> MAAQGFLLIATFLLVLMVLARPLGSGLARLINDIPLPGTTGVERVLFRALGVSDREMNWKQYLCAILGLNMLGLAVLFFMLLG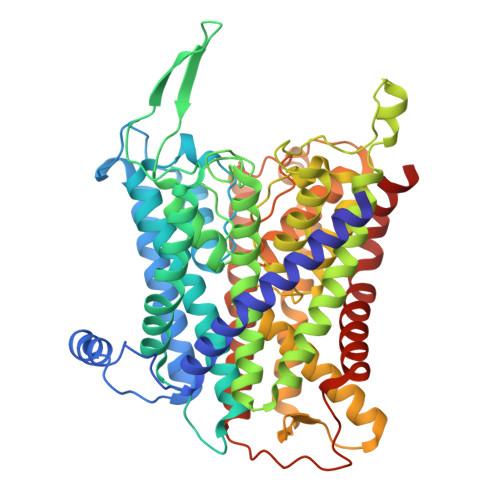QHYLPLNPQQLPGLSWDLALNTAVSFVTNTNWQSYSGETTLSYFSQMAGLTVQNFLSAASGIAVIFALIRAFTRQSMSTLGNAWVDLLRITLWVLVPVALLIALFFIQQGALQNFLPYQAVNTVEGAQQLLPMGPVASQEAIKMLGTNGGGFFNANSSHPFENPTALTNFVQMLAIFLIPTALCFAFGEVMGDRRQGRMLLWAMSVIFVICVGVVMWAEVQGNPHLLALGTDSSINMEGKESRFGVLVSSLFAVVTTAASCGAVIAMHDSFTALGGMVPMWLMQIGEVVFGGVGSGLYGMMLFVLLAVFIAGLMIGRTPEYLGKKIDVREMKLTALAILVTPTLVLMGAALAMMTDAGRSAMLNPGPHGFSEVLYAVSSAANNNGSAFAGLSANSPFWNCLLAFCMFVGRFGVIIPVMAIAGSLVSKKSQAASSGTLPTHGPLFVGLLIGTVLLVGALTFIPALALGPVAEYLS>[2x]GGSLPTAQEVQGLMARYIELVDVGDIEAIVQMYADDATVEDPF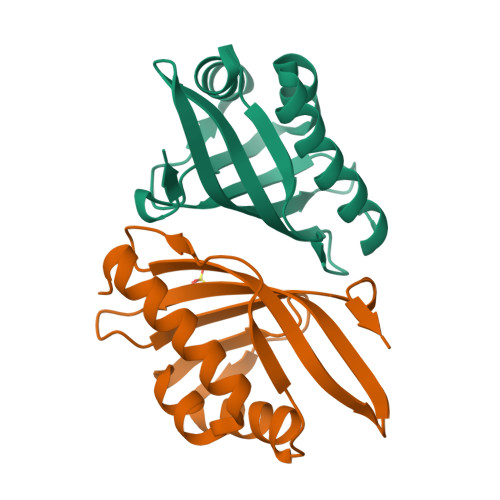GQPPIHGREQIAAFYRQGLGGGKVRACLTGPVRASHNGCGAMPFRVEMVWNGQPCALDVIDVMRFDEHGRIQTMQAYWSEVNLSVREPQ> MGSWRETKLLLIDDNLDRSRDLAVILNFLGEDQLTCNSEDWREVAAGLSNSREALCVLLGSVESKGGAVELLKQLASWDEYLPILLIGEPAPADWPEELRRRVLASLEMPPSYNKLLDSLHRAQVYREMYDQARERGRSREPNLFRSLVGTSRAIQQVRQMMQQVADTDASVLILGESGTGKEVVARNLHYHSKRREGPFVPVNCGAIPAELLESELFGHEKGAFTGAITSRAGRFELANGGTLFLDEIGDMPLPMQVKLLRVLQERTFERVGSNKTQNVDVRIIAATHKNLEKMIEDGTFREDLYYRLNVFPIEMAPLRERVEDIALLLNELISRMEHEKRGSIRFNSAAIMSLCRHDWPGNVRELANLVERLAIMHPYGVIGVG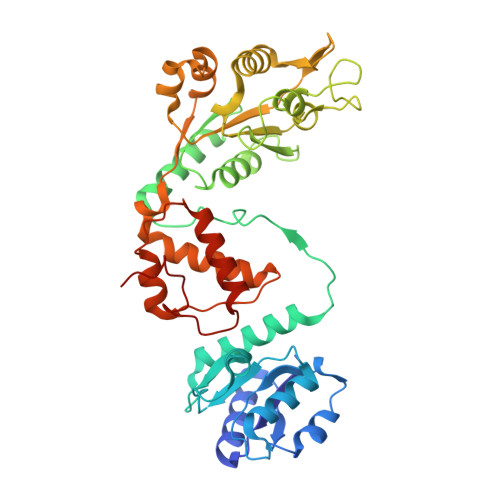ELPKKFRHVD> AKRLTKAHWFEIQHIQPSPLQCNRAMSGINNYTQHCKHQNTFLHDSFQNVAAVCDLLSIVCKNRRHNCHQSSKPVNMTDCRLTSGKYPQCRYSAAAQYKFFIVACDPPQKSDPPY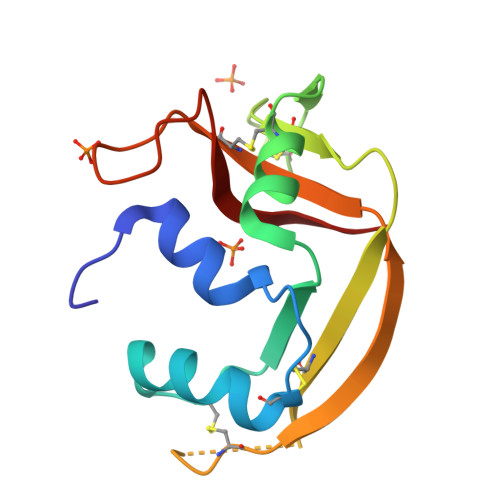KLVPVHLDSIL> TKEGM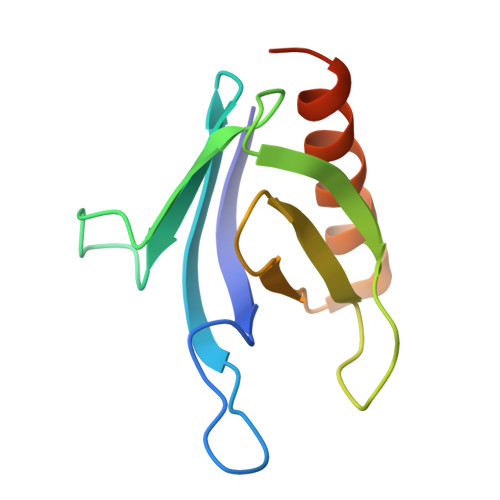LHYKAGTSYLGKEHWKTCFVVLSNGILYQYPDRTDVIPLLSVNMGGEQCGGCRRANTTDRPHAFQVILSDRPCLELSAESEAEMAEWMQHLCQAVSKGVIPQGVAPS>MGVKTFQFPFAEQLEKVAEQFPTFQILNEEGEVVNEEAMPELSDEQLKELMRRMVYTRILDQRSISLNRQGRLGFYAPTAGQEASQIASHFALEKEDFILPGYRDVPQIIWHGLPLYQAFLFSRGHFHGNQIPEGVN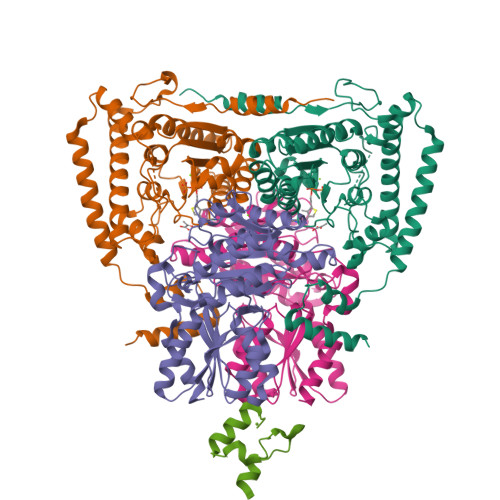VLPPQIIIGAQYIQAAGVALGLKMRGKKAVAITYTGDGGTSQGDFYEGINFAGAFKAPAIFVVQNNRFAISTPVEKQTVAKTLAQKAVAAGIPGIQVDGMDPLAVYAAVKAARERAINGEGPTLIETLCFRYGPHTMSGDDPTRYRSKELENEWAKKDPLVRFRKFLEAKGLWSEEEENNVIEQAKEEIKEAIKKADETPKQKVTDLISIMFEELPFNLKEQYEIYKEKESK[4x];>MAQMTMVQAITDALRIELKNDPNVLIFGEDVGVNGGVFRATEGLQAEFGEDRVFDTPLAESGIGGLAIGLALQGFRPVPEIQFFGFVYEVMDSICGQMARIRYRTGGRYHMPITIRSPFGGGVHTPELHSDSLEGLVAQQPGLKVVIPSTPYDAKGLLISAIRDNDPVIFLEHLKLYRSFRQEVPEGEYTIPIGKADIKREGKDITIIAYGAMVHESLKAAAELEKEGISAEVVDLRTVQPLDIETIIGSVEKTGRAIVVQEAQRQAGIAANVVAEINERAILSLEAPVLRVAAPDTVYPFAQAESVWLPNFKDVIETAKKVMNF[4x];>MAFEFKLPDIGEGIHEGEIVKWFVKPGDEVNEDDVLCEVQNDKAVVEIPSPVKGKVLEILVPEGTVATVGQTLITLDAPGYENMTFKGQEQEEAKKEEKTETVSKEEKVDAVAPNAPAAEAEAGPNRRVIAMPSVRKYAREKGVDIRLVQGTGKNGRVLKEDIDAFLAGGAKPAPAAAEEKAAPAAAKPATTEGEFPETREKMSGIRRAIAKAMVHSKHTAPHVTLMDEADVTKLVAHRKKFKAIAAEKGIKLTFLPYVVKALVSALREYPVLNTSIDDETEEIIQKHYYNIGIAADTDRGLLVPVIKHADRKPIFALAQEINELAEKARDGKLTPGEMKGASCTITNIGSAGGQWFTPVINHPEVAILGIGRIAEKPIVRDGEIVAAPMLALSLSFDHRMIDGATAQKALNHIKRLLSDPELLLMEA[2x]>GSMKKIEAIIRSDKLEDLKAALVQSGFIKGMTISQVLGFGNQRGYTEYVRGQKITPTLLAKVKVEIVAHDAAVEEMITTISQAVKT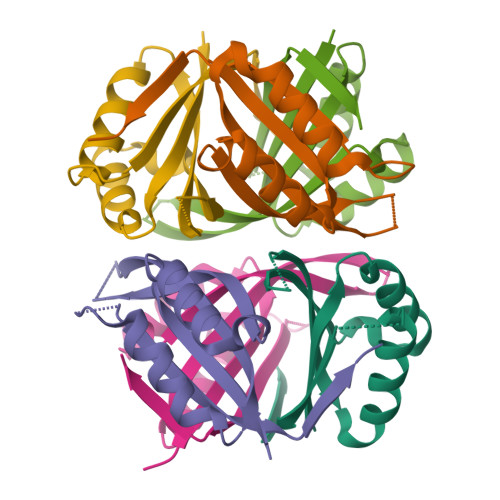GEVGDGKIFVSPVDEIVRIRTGERDGDAI[6x]>MG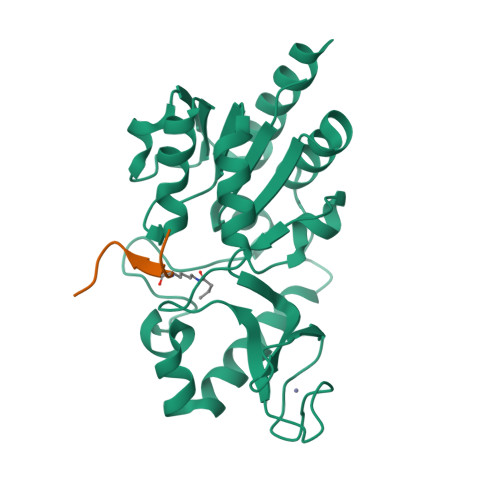SSHHHHHHSQDPKPRVLVLTGAGISAESGIRTFRAADGLWEEHRVEDVGTPEGFDRDPELVQAFYNARRRQLQQPEIQPNAAHLALAKLQDALGDRFLLVTQNCDNLHERAGNTNVIHMHGELLKVRCSQSGQALDWTGDVTPEDKCHCCQFPAPLRPHVVWFGEMPLGMDEIYMALSMADIFIAIGTSGHVYPAAGFVHEAKLHGAHTVELNLEPSQVGNEFAEKYYGPASQVVPEFVEKLLKGLKAGSIA[2x];>[2x]KGGAXRHRKIL We installed thiol-reactive derivatives of the naphthalene-based fluorophore Prodan into bacterial periplasmic glucose-binding proteins. Glucose is bound at the interface between two domains of ecGBP. The protein adopts two conformations that interconvert via bending of a three-stranded β hinge connecting these domains. Glucose binding stabilizes a closed conformation in which the sugar pyranose ring is sandwiched between two aromatic side-chains and surrounded by an annulus of hydrogen bonds between side-chains and glucose hydroxyls.

We determined high-resolution X-ray structures representing the ground states of the two major spectral forms: the glucose complexes of the Blue ttGBP.F17C•Badan and Green ecGBP.W183C•Acrylodan conjugates. In the ecGBP.W183C•Acrylodan glucose complex, the ground-state carbonyl is coplanar with the naphthalene ring and emits a green color when excited, whereas in the ttGBP.F17C•Badan glucose complex it has twisted ~30° out of plane, and emits a blue color upon excitation. In ttGBP.F17C•Badan, the carbonyl hole is formed by D238 and N258. D238 lies within the C-terminal domain and forms hydrogen bonds with the glucose 2- and 3-hydroxyls. N258 is located on one of the hinge strands, and forms a hydrogen bond with the glucose 1-hydroxyl. The Cβ and Cγ atoms of both residues form van der Waals contacts with the twisted carbonyl. Instead, the rings point out of the glucose-binding pocket into the solvent and are each wedged inside a narrow channel (“aromatic channel”) formed within the interface between the N- and C-terminal domains. Each conjugate protrudes through a different channel, located in different parts of the interface, ~120° apart. By contrast, the dimethyl amino (DMA) groups of the fluorophores in these two structures point into solution and are isolated from the surrounding protein. For instance, the D238N mutation in the carbonyl hole of ttGBP.F17C•Acrylodan improves color switching from (ΔλB=−15 nm, ρ*=0.03) to (ΔλB=−29 nm, ρ*=0.21).

> MKQLNIGVAIYKFDDTCMTGVRNAMTAEAQGKAKLNMVDSQNSQPTQNDQVDLFITKKMNALAINPVDRTAAGTIIDKAKQANIPVVFFNREPLPEDMKKWDKVYYVGAKAEQSGILQGQIMADYWKAHPEADKNHDGVMQYVMLMGQPGHQDAILRTQYSIQTVKDAGIKVQELAKDYANWDRVTAHDKMAAWLSSFGDKIEAVFANNDDMALGAIEALKSAGYFTGNKYIPVVGVDATAPGIQAIKDGTLLGTVLNDAKNQAKATFNIAYELAQGITPTKDNIGYDITDGKYVWIPYKKITKDNISDAE> MTSKVYDPEQRKRMITGPQWWARCKQMNVLDSFINYYDSEKHAENAVIFLHGNATSSYLWRHVVPHIEPVARCIIPDLIGMGKSGKSGNGSYRLLDHYKYLTAWFELLNLPKKIIFVGHDWGAALAFHYAYEHQDRIKA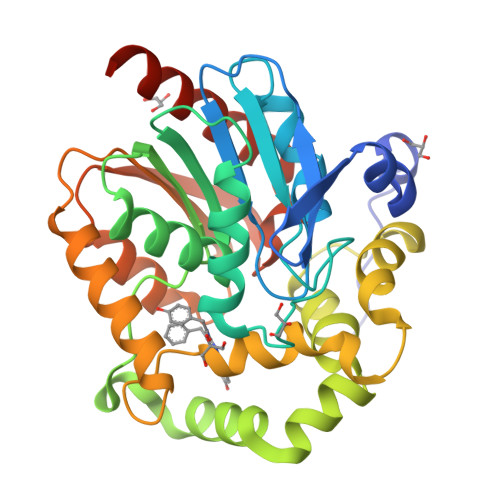IVHMESVVDVIESWDEWPDIEEAIALIKSEEGEKMVLENNFFVETVLPSKIMRKLEPEEFAAYLEPFKEKGEVRRPTLSWPREIPLVKGGKPDVVQIVRNYNAYLRASDDLPKLFIESDPGFFSNAIVEGAKKFPNTEFVKVKGLHFLQEDAPDEMGKYIKSFVERVLKNEQHHHHHH> MTTRPAESAPQTASTLLEPGSNGVVRLLGGPGTGKSSLLVDTAVQHILAGADPESVLLLTGSARLRTAARAAITARLLGAGTVGVVREPLVRTVHSYAFAVLRLAAQRNGDPPPRLITSAEQDGIIRELLAGDLEDGHRSPVGWPEQLWPALTTAGFATELRDLMARCTERGVDPIALQRLGRTAKRPEWLAAGRFAQAYEQIMLLRSAVGMAAPQATVPALGAAELVGAALEALGADDELLDTERNRIKLLLVDDAQHLDPQAARLVRALAAGTGLTVIAGDPDQSVFGYRGADPVLLRDDTHPAITLTQSYRCAPEIASAITGLGQRLPGVSDTRHWTGNPQREGTVTVRLAASTHAEGTMIADALRRAHLVDGIPWSQMAVIVRSVPRVGTALARALTAAGVPVQDNGTDVPVGRQPAAAALLTVLDVTATGHLDADSAVALLTGPIGRVDPVTLRQLRRALRRADGSQPPRDFGDLLVDAIEREPKGLSAEHARTLRRLRAVLTAARRSDASGADPRYTLWQAWHASGLQRRWLAASERGGSVGAQADRDLDAVTTLFDVADQYVNRTAGASLRGLVDHVTRLGAAVARTEPETAAEAVAVLSVHGALAGEWDFVVIAGVQEGLWPNMIPRGGV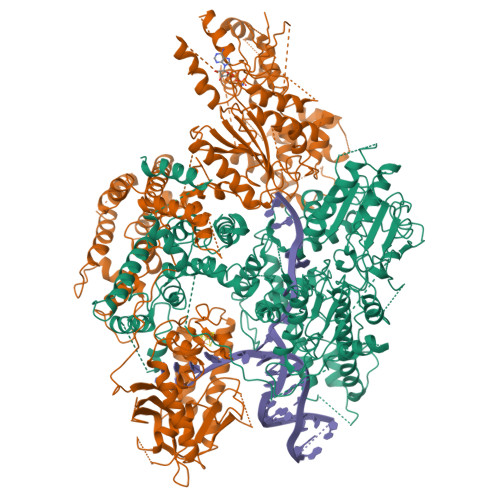LGTQHLVDVLDGVADMTDRTVSTRAPLVAEERRLLMAAMGRARTRVMITAVDSDTGDESLLPSPFCAEISAWATEPVAEPPLVAPRVLAPSALVGRLRAVVCAPDGAVDDDARACAAAQLARLAAAGVPGADPSQWHAMTSLTTEEPLWSEPGHVVTLSPSTLQMLTDCPLRWLLERHGGDDGRDVRSTVGSLVHALVSEPGKTESQLVNELEKVWDDLPYDAKWYSDNELARHRAMLETFTRWREDTRRQLTEVATEIPVEGIVVEPGENTPGVRVRGRLDRLERDEAGRLVVVALKTGKSPVTKDDAQNHAQLAMYQLAVAAGLLDDGDEPGGGKLVYLGKAGAAGATEREQDPLTPDKRAEWLETVGEAAAATAGPRFVARVNNGCANCPVRSSCPAQANGDRP;> MTQVASPVVQARYSPVELSAALGLFPPTDEQAAVIAAPPGPLVVIAGAGAGKTETMAARVVWLVANGFATPSQVLGLTFTRKAAGQLLRRVRTRLARLAGAGLAPGSGASDESATVSTYHAFAGTLLREHGLLLPVEPDTRLLSETELWQLAYDVVCAHPGHLDTEKTPAAVTAMVLRLSGALAEHLVDTDQLRDTHVELERLVHTLPAGPYQRDRGPSQWLLRMLATQTERTELVPLIDALHQRMRAEKVMDFGMQMAAAARLAARFPQVGEQLRQRFRVVLLDEYQDTGHAQRIALSSLFGGGADDGLALTAVGDPIQSIYGWRGASATNLPRFTTDFPYSDGTPAPTLELRTSWRNPPSTLHVANAVSEEARRRSVAVRALRPRPDAEPGTIRCALLNNVAAERDWVADHLARAYHGAIGRGEAAPTAAVLVRRNADAAPMAEALTARGVPVEVVGVAGLLAVPEVADLVAMLRLIADPTAGSAVMRILTGPRWRFGARDIAALWRRAVELDDRPKGELGTADIVAQAAPDADTACVADAICDPGDAERYSPAGYERIVALGRELTMLRAHLGHPLPELVAEVRRVLGLDAEARAARPVAAGWAGTENLDRFSDLVSDFAGHAGASVSALLAYLDAAVEVENGLAPAELTVSHDRVQILTVHAAKGLEWQVVAVPHLSARVFPSTTQARTWLTDASDLPPLLRGDRATESEIGVPVLDTSDIYDRKILSDKISDHKKSLDQRRVDEERRLLYVAITRAEDTLLLSGHHWGATESKPRGPSEFLCELKTILEEATAAGTPCGEIEHWAPDPAPGETNPLRDQVVEALWPPVASADDHVHRGAQLVAAAMAGEVSAEADQEGWAADVDALLAERERPPQQEDTELPGQLSVSTLVELSRDPKAALTRLRRRLPQRPDPHALLGTTFHEWVQRYFHAERLFDLDDLPGAVDSDSGRAVEESLAELQDAFVKSPWAARTPVEVEVPFDMVLGETVVRGRIDAVFAEPDGTTMVLAWKTGDPPETPEAKEHAAVQLAVYRLAWAAMRGCPPESVRAAFHYVRSGQTVIPETLPGAEELVKLLAAAPTETAEEADRIT> MDATRTFFGLPNVHNVPLCLTSNLSLFPQRLLQKHTLPLKPAKKHHLVCVRSTKSSDDLEGSRPSTYFSPSLWGDHFLSVSLDRGEFDELEREIETMKPLVKDMLMSSQSSDKEKIRLIHLLVSLGSSYHFDKEIQDILKHSFTKLDDIIVGEDDLETISIMFEVFRLYGHKMSCDAFDRFRGEDGRFKESLAKDVRGMLQLFEVAHLGTPSEDIMDEASSFAQNHLDSWIGGNVSGATPHLLKHIQNSLYIPRYCNIEVLVAREYISYYEQ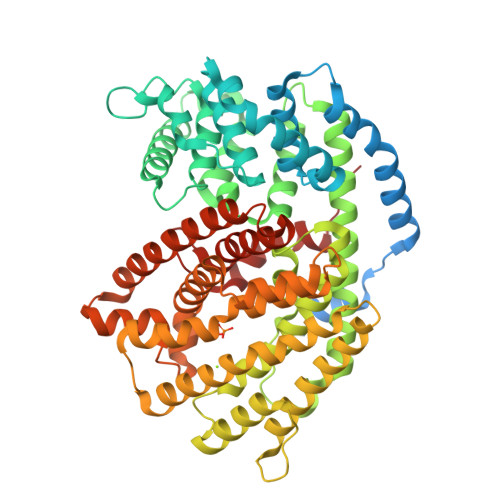EEGHNKILLKFAKLNFNFCQFHYIQELKTLTKWWKDLDLASKLPYIRDRLVESHLGGLGPYFEPHYSLGRIIVAKIIMTMVVVDDTYDAHATVPEVAVLTECLQRLNIGADDKLPDYLRTVLESVFEVMGEIEQEMRPKGRSYGVKQVLERFKNVAKADKQLTEWARTGDVPSFDEYMKVGLVTAGMDGYAGYCFIGMEDVSEKEAFEWLSSNPLIIQALNVMFRLANDVGTYETEINRGEVANGLNCYMKQYGVTKEEASQELRKIYSNNKKVVMEEFMNSHDHVPRQVLLRCLNFARLFDVMYTEGDGYSEPKGKIEHFMTSLYVHPIPLS> FDVGDEYEIIETIGNGAYGVVSSARRRLTGQQVAIKKIPNAFDVVTNAKRTLRELKILKHFKHDNIIAIKDILRPTVPYGEFKSVYVVLDLMESDLHQIIHSSQPLTLEHVRYFLYQLLRGLKYMHSAQVIHRDLKPSNLLVNENCELKIGDFGMARGLCTSPAEHQY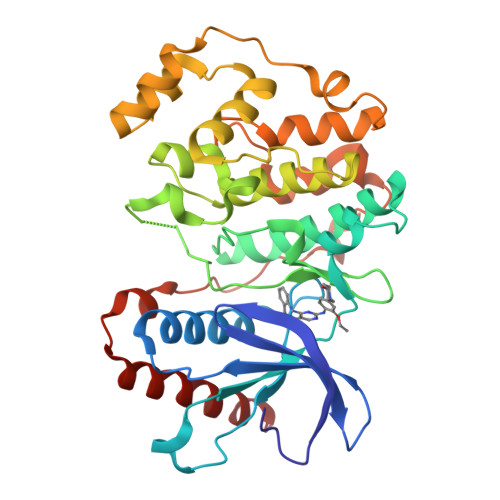FMTEYVATRWYRAPELMLSLHEYTQAIDLWSVGCIFGEMLARRQLFPGKNYVHQLQLIMMVLGTPSPAVIQAVGAERVRAYIQSLPPRQPVPWETVYPGADRQALSLLGRMLRFEPSARISAAAALRHPFLAKYHDPDDEPDCAPPFDFAFDREALTRERIKEAIVAEIEDFHARREG> QAADDRQLLIRIKRVWRDPPVLAAWNGSGDHCTWPYVTCDASGRVTSLSLANTGVAGPFPDAIGGLSGLTSLDLSGNYLDGELPADIGRALGKNLTSLMLNGNYFNGTIPTSLSRLKNLQSLALDNNFLAGTIPAELGDLTGLQMLTLANNSFSVGVLPASFKNLTQLKTFWAAICNLTGDFPSYVAEMRELEVLDLSVNALTGSIPPAIWNLAKLQTMALFANNFTGGVVVADGAFSAVNLVMIDLSSNHRLSGPIPEAFGHLPNLETLNLYFNNFSGEIPASIGRLPSLVTLSLFRNRLTGRLPPDLGKNSSAGLMYIDVDDNEISGAIPEGLCANGKFQSLIARNNRLNGSIPAGLASCATLNNLMLGNNQLSGEVPEALWTVPQLEYVLLRNNRLSGSLPVKMFINLSTLHIENNQFGGNIPAAAVGLREFIAGNNNFSGEMPASLGKGMPLLQAMNLSGNQLFGGIPSSVAKLRLLTQLDLSRNQLAGEIPAELGAMRVLSALDLSSNKLSGYIPPPLAGLPLTFLNLSSNQLDGQVPAGLATAAYDRSFLGNPGLCHAGLGPRYLTGVRSCAAGS;> NTEGDALYSLRQSLKDANNVLQSWDPTLVNPCTWFHVTCNTDNSVIRVDLGNAQLSGALVSQLGQLKNLQYLELYSNNISGTIPLELGNLTNLVSLDLYLNKFTGGIPDTLGKLLKLRFLRLNNNSLSGQIPQSLTNISTLQVLDLSNNNLSGAVPSTGSFSLFTPISFGNNPNLCGPGTTKPCPGA;> 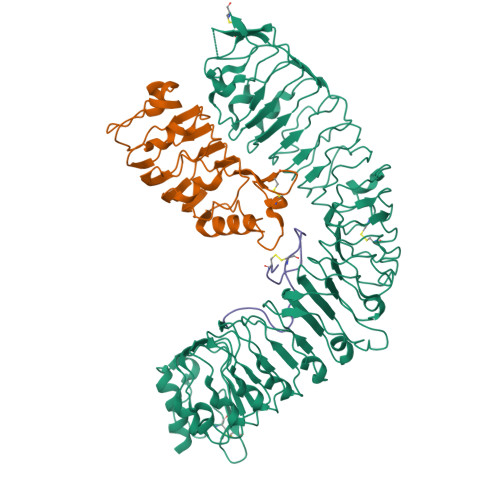PRGGGSAGAPNGCTNNPKHPPGGKCHG N-(4-{[(3R)-3-[(biphenyl-4-ylsulfonyl)(propan-2-yloxy)amino]-4-(hydroxyamino)-4-oxobutyl]amino}-4-oxobutyl)-N'-(4-{[(3S)-3-[(biphenyl-4-ylsulfonyl)(propan-2-yloxy)amino]-4-(hydroxyamino)-4-oxobutyl]amino}-4-oxobutyl)benzene-1,3-dicarboxamide 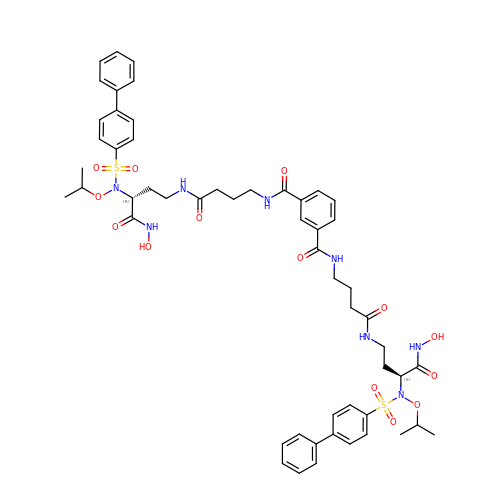| C54 H66 N8 O14 S2 | QTGQZAQZBAEHLR-WPVYDPPMSA-N> MTASELVAGDLAGGRAPGALPLDTTWHRPGWTIGELEAAKAGRTISVVLPALNEEATIESVIDSISPLVDGLVDELIVLDSGSTDDTEIRAIASGARVVSREQALPEVPVRPGKGEALWRSLAATSGDIVVFIDSDLINPHPLFVPWLVGPLLTGEGIQLVKSFYRRPLQVSDVTSGVCATGGGRVTELVARPLLAALRPELGCVLQPLSGEYAASRELLTSLPFAPGYGVEIGLLIDTFDRLGLDAIAQVNLGVRAHRNRPLDELGAMSRQVIATLLSRCGIPDSGVGLTQFLPGGPDDSDYTRHTWPVSLVDRP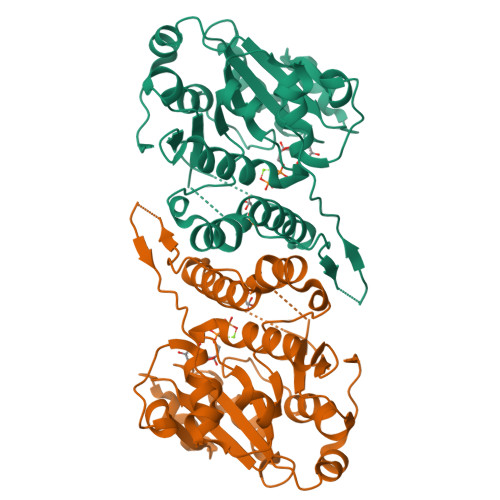PMKVMRPRKLAAALEHHHHHH> DKMDYDFKVKLSSERERVEDLFEYEGCKVGRGTYGHVYKAKRKDGKDDKDYALKQIEGTGISMSACREIALLRELKHPNVISLQKVFLSHADRKVWLLFDYAEHDLWHIIKFHRASKANKKPVQLPRGMVKSLLYQILDGIHYLHANWVLHRDLKPANILVMGEGPER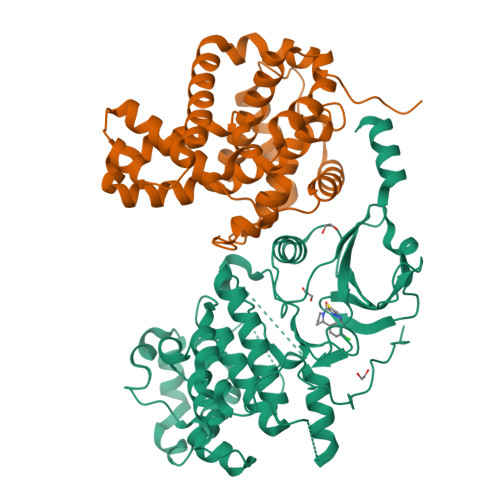GRVKIADMGFARLFNSPLKPLADLDPVVVTFWYRAPELLLGARHYTKAIDIWAIGCIFAELLTSEPIFHCRQEDIKTSNPYHHDQLDRIFNVMGFPADKDWEDIKKMPEHSTLMKDFRRNTYTNCSLIKYMEKHKVKPDSKAFHLLQKLLTMDPIKRITSEQAMQDPYFLEDPLPTSDVFAGCQIPYPKREFLTEE;> DKAMAGNFWQSSHYLQWILDKQDLLKERQKDLKFLSEEEYWKLQIFFTNVIQALGEHLKLRQQVIATATVYFKRFYARYSLKSIDPVLMAPTCVFLASKVEEFGVVSNTRLIAAATSVLKTRFSYAFPKEFPYRMNHILECEFYLLELMDCCLIVYHPYRPLLQYVQDMGQEDMLLPLAWRIVNDTYRTDLCLLYPPFMIALACLHVACVVQQKDARQWFAELSVDMEKILEIIRVILKLYEQWKNFDERKEMATILSKMPKPKPPP> GSSSTAATSRDALPNTEASGPTHSKEIPALTAVETGATNPLVPSDTVQTRHVVQHRSRSESSIESFFARGACVTIMTVDNPASTTNKDKLFAVWKITYKDTVQLRRKLEFFTYSRFDMELTFVVTANFTETNNGHALNQVYQIMYVPPGAPVPEKWDDYTWQTSSNPSIFYTYGTAPARISVPYVGISNAYSHFYDGFSKVPLKDQSAALGDSLYGAASLNDFGILAVRVVNDHNPTKVTSKIRVYLKPKHIRVWCPRPPRAVAYYGPGVDYKDGTLTPLSTKDLTTY;> EACGYSDRVLQLTLGNSTITTQEAANSVVAYGRWPEYLRDSEANPVDQPTEPDVAACRFYTLDTVSWTKESRGWWWKLPDALRDMGLFGQNMYYHYLGRSGYTVHVQCNASKFHQGALGVFAVPEMCLAGDSNTTTMHTSYQNANPGEKGGTFTGTFTPDNNQTSPARRFCPVDYLLGNGTLLGNAFVFPHQIINLRTNNCATLVLPYVNSLSIDSMVKHNNWGIAILPLAPLNFASESSPEIPITLTIAPMCCEFNGLRNITLPRLQ;> GLPVMNTPGSNQYLTADNFQSPC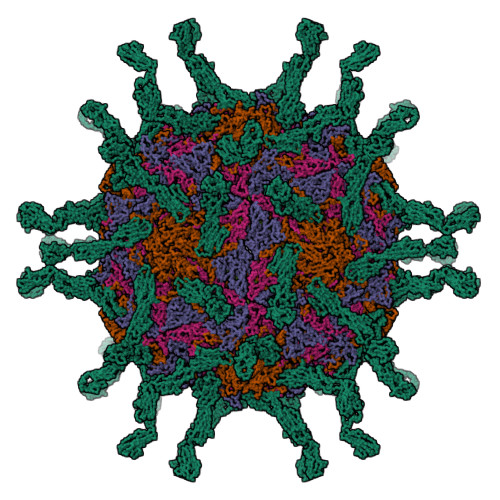ALPEFDVTPPIDIPGEVKNMMELAEIDTMIPFDLSATKKNTMEMYRVRLSDKPHTDDPILCLSLSPASDPRLSHTMLGEILNYYTHWAGSLKFTFLFCGSMMATGKLLVSYAPPGADPPKKRKEAMLGTHVIWDIGLQSSCTMVVPWISNTTYRQTIDDSFTEGGYISVFYQTRIVVPLSTPREMDILGFVSACNDFSVRLLRDTTHIEQKA;> XGAQVSSQKVGAHENSSTINYTTINYYRDSASNAASKQDFSQDPSKFTEPIKDVLIKTAPMLN;> DVVVQAPTQVPGFLGDSVTLPCYLQVPNMEVTHVSQLTWARHGESGSMAVFHQTQGPSYSESKRLEFVAARLGAELRNASLRMFGLRVEDEGNYTCLFVTFPQGSRSVDIWLRVLAKPQNTAEVQKVQLTGEPVPMARCVSTGGRPPAQITWHSDLGGMPNTSQVPGFLSGTVTVTSLWILVPSSQVDGKNVTCKVEHESFEKPQLLTVNLTVYYPPEVSISGYDNNWYLGQNEATLTCDARSNPEPTGYNWSTTMGPLPPFAVAQGAQLLIRPVDKPINTTLICNVTNALGARQAELTVQV~{N}-methyl-1-(3-thiophen-2-ylphenyl)methanamine | C12 H13 N S | 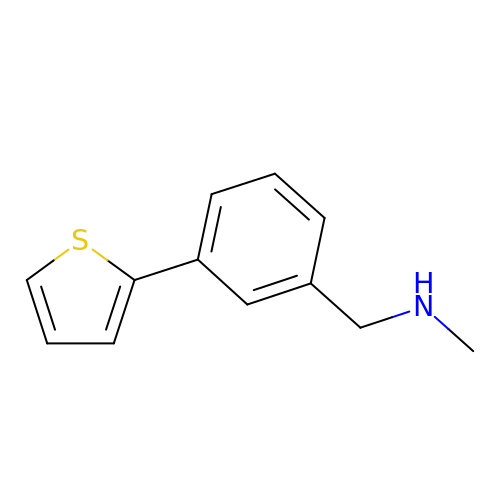BIULJOFRQMLCQK-UHFFFAOYSA-N> MAKMRISPELKKLIEKYRCVKDTEGMSPAKVYKLVGENENLYLKMTDSRYKGTTYDVEREKDMMLWLEGKLPVPKVLHFERHDGWSNLLMSEADGVLCSEEYEDEQSPEKIIELYAECIRLFHSIDISDCPYTNSLDSRLAELDYLLNNDLADVDCENWEEDTPFKDPRELYDFLKTEKPEEELVFSHGDLGDSNIFVKDGKVSGFIDLGRSGRADKWYDIAFCVRSIREDIGEEQY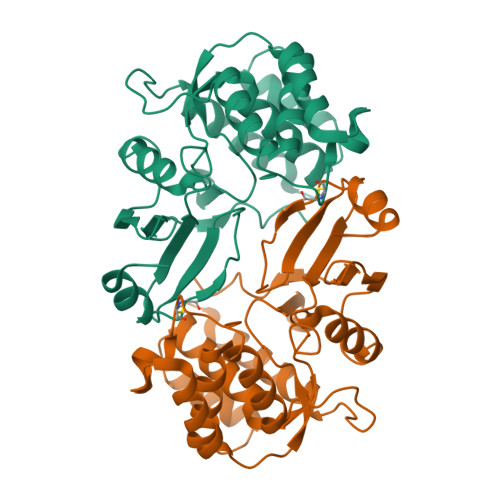VELFFDLLGIKPDWEKIKYYILLDELF> EGKSEFAENDAYVHATPLIRRLAREFGVNLAKVKGTGRKGRILREDVQAYVKEAIKRAEAAPAATG;>SERFPNDVDPIETRDWLQAIESVIREEGVERAQYLIDQLLAE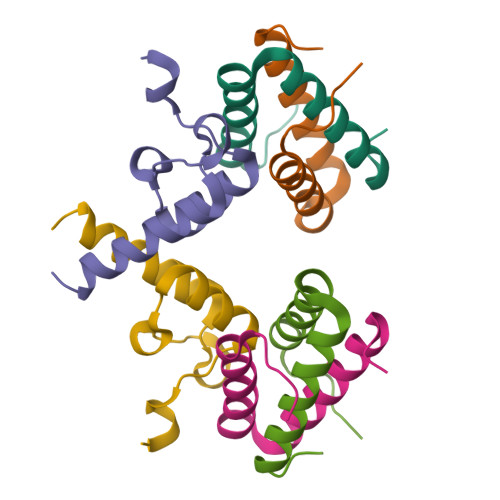ARKGGVN[2x]> GGSGGSMPPPADIVKVAIEWPGAYPKLMEIDQKKPLSAIIKEVCDGWSLANHEYFALQHADSSNFYITEKNRNEIKNGTILRLTTSPAQNAQQLHERIQSSSMDAKLEALKDLASLSRDVTFAQEFINLDGISLLTQMVESGTERYQKLQKIMKPCFGDMLSFTLTAFVELMDHGIVSWDTFSVAFIKKIASFVNKSAIDISILQRSLAILESMVLNSHDLYQKVAQEITIGQLIPHLQGSDQEIQTYTIAVINALFLKAPDERRQEMANILAQKQLRSIILTHVIRAQRAINNEMAHQLYVLQVLTFNLLEDRMMTKMDPQDQAQRDIIFELRRIAFDAESEPNNSSGSMEKRKSMYTRDYKKLGFINHVNPAMDFTQTPPGMLALDNMLYFAKHHQDAYIRIVLENSSREDKHECPFGRSSIELTKMLCEILKVGELPSETCNDFHPMFFTHDRSFEEFFCICIQLLNKTWKEMRATSEDFNKVMQVVKEQVMRALTTKPSSLDQFKSKLQNLSYTEILKIRQSERMNQEDFQSRPILELKEKIQPEILELIKQQRLNRLVEGTCFRKLNARRRQDKFWYCRLSPNHKVLHYGDLEESPQGEVPHDSLQDKLPVADIKAVVTGKDCPHMKEKGALKQNKEVLELAFSILYDSNCQLNFIAPDKHEYCIWTDGLNALLGKDMMSDLTRNDLDTLLSMEIKLRLLDLENIQIPDAPPPIPKEPSNYDFVYDCN;>GGSGGSMARWIPTKRQKYGVAIYNYNASQDVELSLQIGDTVHILEMYEGWYRGYTLQNKSKKGIFPETYIHLKEATVEDLGQHETVIPGELPLVQELTSTLREWAVIWRKLYVNNKLTLFRQLQQMTYSLIEWRSQILSGTLPKDELAELKKKVTAKIDHGNRMLGLDLVVRDDNGNILDPDETSTIALFKAHEVASKRIEEKIQEEKSILQNLDLRGQSIFSTIHTYGLYVNFKNFVCNIGEDAELFMALYDPDQSTFISENYLIRWGSNGMPKEIEKLNNLQAVFTDLSSMDLIRPRVSLVCQIVRVGHMELKEGKKHTCGLRRPFGVAVMDITDIIHGKVDDEEKQHFIPFQQIAMETYIRQRQLIMSPLITSHVIGENEPLTSVLNKVIAAKEVNHKGQGLWVSLKLLPGDLTQVQKNFSHLVDRSTAIARKMGFPEIILPGDVRNDIYVTLIHGEFDKGKKKTPKNVEVTMSVHDEEGKLLEKAIHPGAGYEGISEYKSVVYYQVKQPCWYETVKVSIAIEEVTRCHIRFTFRHRSSQETRDKSERAFGVAFVKLMNPDGTTLQDGRHDLVVYKGDNKKMEDAKFYLTLPGTKMEMEEKELQASKNLVTFTPSKDSTKDSFQIATLICSTKLTQNVDLLGLLNWRSNSQNIKHNLKKLMEVDGGEIVKFLQDTLDALFNIMMEMSDSETYDFLVFDALVFIISLIGDIKFQHFNPVLETYIYKHFSATLAYVKLSKVLNFYVANADDSSKTELLFAALKALKYLFRFIIQSRVLYLRFYGQSKDGDEFNNSIRQLFLAFNMLMDRPLEEAVKIKGAALKYLPSIINDVKLVFDPVELSVLFCKFIQSIPDNQLVRQKLNCMTKIVESTLFRQSECREVLLPLLTDQLSGQLDDNSNKPDHEASSQLLSNILEVLDRKDVGATAVHIQLIMERLLRRINRTVIGMNRQSPHIGSFVACMIALLQQMDDSHYSHYISTFKTRQDIIDFLMETFIMFKDLIGKNVYAKDWMVMNMTQNRVFLRAINQFAEVLTRFFMDQASFELQLWNNYFHLAVAFLTHESLQLETFSQAKRNKIVKKYGDMRKEIGFRIRDMWYNLGPHKIKFIPSMVGPILEVTLTPEVELRKATIPIFFDMMQCEFNFSGNGNFHMFENELITKLDQEVEGGRGDEQYKVLLEKLLLEHCRKHKYLSSSGEVFALLVSSLLENLLDYRTIIMQDESKENRMSCTVNVLNFYKEKKREDIYIRYLYKLRDLHRDCENYTEAAYTLLLHAELLQWSDKPCVPHLLQRDSYYVYTQQELKEKLYQEIISYFDKGKMWEKAIKLSKELAETYESKVFDYEGLGNLLKKRASFYENIIKAMRPQPEYFAVGYYGQGFPSFLRNKIFIYRGKEYERREDFSLRLLTQFPNAEKMTSTTPPGEDIKSSPKQYMQCFTVKPVMSLPPSYKDKPVPEQILNYYRANEVQQFRYSRPFRKGEKDPDNEFATMWIERTTYTTAYTFPGILKWFEVKQISTEEISPLENAIETMELTNERISNCVQQHAWDRSLSVHPLSMLLSGIVDPAVMGGFSNYEKAFFTEKYLQEHPEDQEKVELLKRLIALQMPLLTEGIRIHGEKLTEQLKPLHERLSSCFRELKEKVEKHYGVITL[2x]

The dedicator of cytokinesis (DOCK)/engulfment and cell motility (ELMO) complex serves as a guanine nucleotide exchange factor (GEF) for the GTPase Rac. RhoG, another GTPase, activates the ELMO-DOCK-Rac pathway during engulfment and migration. The DOCK-A (DOCK1/2/5) and DOCK-B (DOCK3/4) subfamilies specifically activate Rac and have an Src homology domain at their N-terminus; the Src homology domain is involved in autoinhibition and binding to engulfment and cell motility (ELMO) scaffold proteins. ELMO is structurally divided into two domains: an N-terminal domain (NTD), consisting of the Ras-binding (RBD), ELMO inhibitory (EID), and ELMO domains, and a C-terminal domain (CTD), consisting of the Pleckstrin homology (PH) domain and proline-rich region.

We initially determined the cryo-EM structure of the DOCK5/ELMO1 binary complex using human full-length DOCK5 (DOCK5FL, residues 1−1870) and ELMO1 (ELMO1FL, residues 1−727) proteins. We next analyzed a DOCK5FL/ELMO1FL sample crosslinked with bis(sulfosuccinimidyl)suberate (BS3), a widely used N-hydroxysuccinimide ester-based crosslinking agent, achieving a reconstruction at improved resolution (5.8 Å) that clearly showed the ELMO1NTD density with two-fold symmetry. To enhance local resolution, we symmetrically expanded and refined the particles, focusing on a single DOCK5/ELMO1 protomer and the dimerization component, which led to structure determination at 4.8 Å resolution. Model building and refinement of the DOCK5FL/ELMO1FL complex were completed, with the exception of the C-terminal region of DOCK5 (residues 1643−1870), which remained disordered. The structure of DOCK5/ELMO1 showed a closed conformation similar to that reported for DOCK2/ELMO1 (21). The α-solenoid of ELMO1NTD was clamped onto the DHR-2 domain of DOCK5, occluding the Rac1 binding site. This indicates that the DOCK1−5/ELMO1 complexes likely have autoinhibitory regulation in common. Despite the common closed conformation, a detailed structural comparison revealed that DOCK5/ELMO1 is more compact than DOCK2/ELMO1, with the two ELMO1 NTDs located closer to each other. A closer interaction was observed for DOCK5 than for DOCK2 at the ELMO1RBD-DHR-2 interface, between Glu36 and Asp39 in ELMO1 and His1545 in DOCK5. The C2 domain of DOCK5 interacted with the ELMO domain of ELMO1 in the apo state of DOCK5/ELMO1.>MMKRNILAVIVPALLVAGTANAAEIYNKDGNKVDLYGKAVGLHYFSKGNGENSYGGNGDMTYARLGFKGETQINSDLTGYGQWEYNFQGNNSEGADAQTGNKTRLAFAGLKYADVGSFDYGRNYGVVYDALGYTDMLPEFGGDTAYSDDFFVGRVGGVATYRNSNFFGLVDGLNFAVQYLGKNERDTARRSNGDGVGGSISYEYEGFGIVGAYGAADRTNLQEAQPLGNGKKAEQWATGLKYDANNIYLAANYGETRNATPITNKFT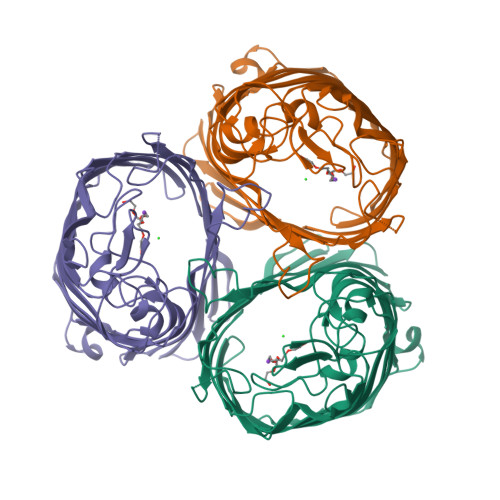NTSGFANKTQDVLLVAQYQFDFGLRPSIAYTKSKAKDVEGIGDVDLVNYFEVGATYYFNKNMSTYVDYIINQIDSDNKLGVGSDDTVAVGIVYQF[2x]>[4x]MAHHHHHHMNQDQLKQAVAQAAVDHILPHLDSKSIVGVGTGSTANFFIDALARHKAEFDGAVASSEATAKRLKEHGIPVYELNTV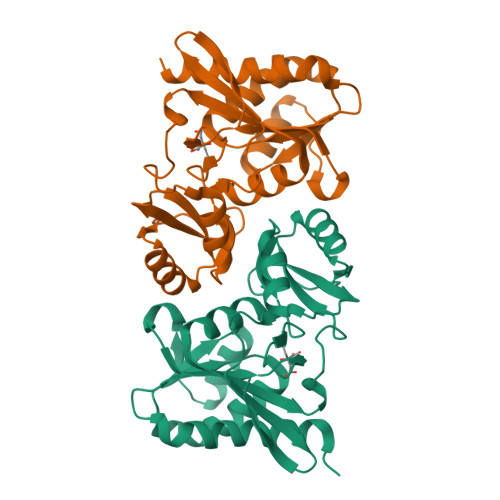SELEFYVDGADESNERLELIKGGGAALTREKIVAAVAKTFICIADASKLVPILGQFPLPVEVIPMARSHVARQLVKLGGDPVYREGVLTDNGNIILDVHNLRIDSPVELEEKINAIVGVVTNGLFAARPADLLLLGTADGVKTLKA> GSHMEKIIIYGGTGYIGKFMVRASLSFSHPTFIYARPLTPDSTPSSVQLREEFRSMGVTIIEGEMEEHEKMVSVLKQVDIVISALPF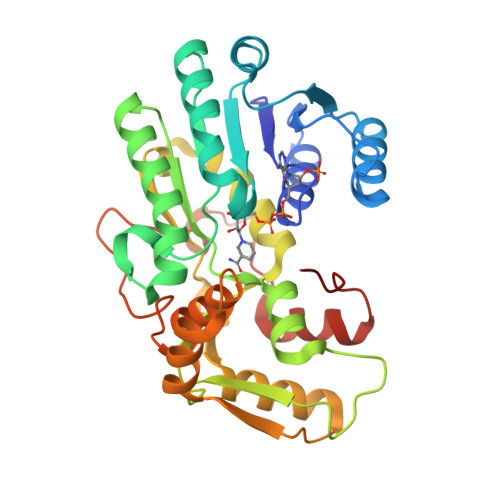PMISSQIHIINAIKAAGNIKRFLPSDFGCEEDRIKPLPPFESVLEKKRIIRRAIEAAALPYTYVSANCFGAYFVNYLLHPSPHPNRNDDIVIYGTGETKFVLNYEEDIAKYTIKVACDPRCCNRIVIYRPPKNIISQNELISLWEAKSGLSFKKVHMPDEQLVRLSQELPQPQNIPVSILHSIFVKGDLMSYEMRKDDIEASNLYPELEFTSIDGLLDLFISGRAPPPTLAEFE> DNKINIGLAVMKILESWGADTIYGIPSGTLSSLMDAMGEEENNVKFLQVKHEEVGAMAAVMQSKFGGNLGVTVGSGGPGASHLINGLYDAAMDNIPVVAILGSRPQRELNMDAFQELNQNPMYDHIAVYNRRVAYAEQLPKLVDEAARMAIAKRGVAVLEVPGDFAKVEIDNDQWYSSANSLRKYAPIAPAAQDIDAAVELLNNSKRPVIYAGIGTMGHGPAVQELARKIKAPVITTGKNFETFEWDFEALTGSTYRVGWKPANETILEADTVLFAGSNFPFSEVEGTFRNVDNFIQIDIDPAMLGKRHHADVAILGDAALAIDEILNKVDAVEESAWWTANLKNIANWREYINMLETKEEGDLQFYQVYNAINNHADEDAIYSIDVGNSTQTSIRHLHMTPKNMWRTSPLFATMGIAIPGGLGAKNTYPDRQVWNIIGDGAF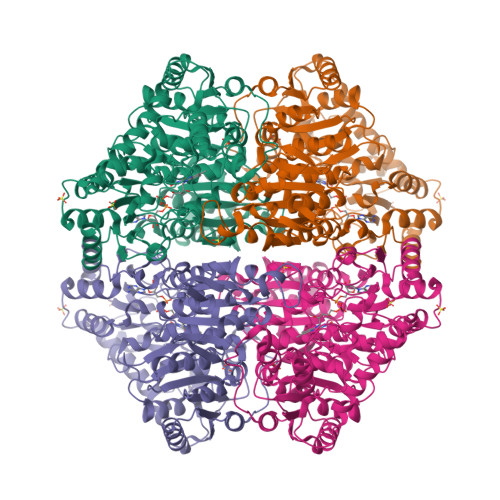SMTYPDVVTNVRYNMPVINVVFSNTEYAFIKNKYEDTNKNLFGVDFTDVDYAKIAEAQGAKGFTVSRIEDMDRVMAEAVAANKAGHTVVIDCKITQDRPIPVETLKLDSKLYSEDEIKAYKERYEAANLVPFREYLEAEGLESKYIK>PSQMEHAMETMMFTFHKFAGDK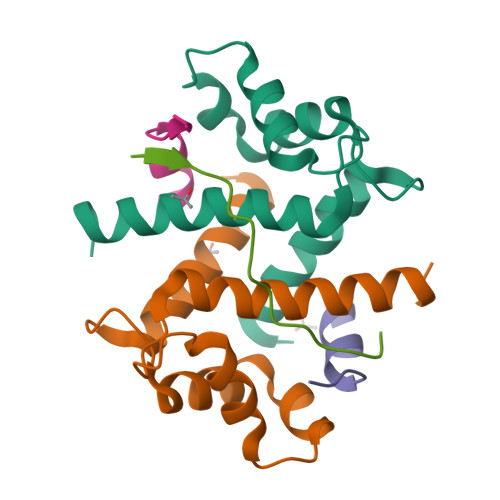GYLTKEDLRVLMEKEFPGFLENQKDPLAVDKIMKDLDQCRDGKVGFQSFFSLIAGLTIACNDYFVVHMKQKGKK[2x];>[2x]XSTVHEILSKLSLEGDX;> XGKVTFPKMKIPKFTFSGRELX> MKDNPPPSTDEIAKAALVGVYNNTQDINGFKVGDTIYDIENGQPKGRPATEDDVKA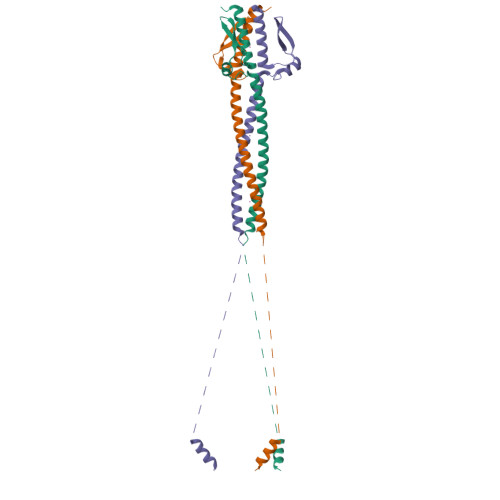DDFGGLGLKEVLAQHDQSLADLTGTVEENSEALVKTAEVVNDISADVKANTAAIRENKAAIATKADKTELDEVSGKVTANETAIGKKANSADVYTKAEVYTKQESDNRFVKIGDRIGNLNTTANGLETRLADAEKSVKDHGTRASKHHHHHH Coxsackievirus A16 (CVA16), a member of the Enterovirus genus within the Picornaviridae family, is one of the major causative agents of hand, foot and mouth disease (HFMD) prevalent in infants and young children. Like other enteroviruses (EVs), CVA16 is a nonenveloped virus of ~30 nm in diameter with a single-stranded, positive-sense RNA genome of ~7.4 kb in length packaged in a protein shell termed capsid. Specifically, CVA16 utilizes cell surface heparan sulfate (HS) glycosaminoglycans as its attachment receptor, and human scavenger receptor B2 (SCARB2, also known as lysosomal integral membrane protein 2, LIMP-2) as its uncoating receptor. Cryo-EM studies show that 9B5 and 8C4 target distinct epitopes located at the 5-fold and 3-fold protrusions of CVA16 capsids, respectively, and exhibit differential binding preference to three forms of naturally occurring CVA16 particles.

From the same CVA16–8C4 dataset, we deduced three conformational states, namely C1, C2, and C3, at the resolution of 3.05, 2.91, and 3.36 Å and population distribution 15.5%, 27.0%, and 57.5%, respectively. For CVA16–8C4 C3, the radius of viral capsid is 170.5 Å, slightly larger than that of C1 and C2 (162.2 and 163.0 Å, respectively), and the two-fold axis channel in its capsid is open, while that in C1 and C2 capsid is closed. Moreover, the VP1 hydrophobic pocket is empty and collapsed in C3 capsid, but filled with the pocket factor in C1 and C2 capsids. Additionally, the viral RNA density is present in C1 but absent in C2 and C3. Collectively, these data suggested that the viral particles in C1, C2, and C3 adopt the native/compact mature CVA16 virion, the compact empty particle, and the expanded empty particle configuration, respectively. Moreover, structural comparison revealed that the protomers of the CVA16–8C4 C1/C2/C3 showed the most similar architecture to that of mature virion, compact empty particle, and expanded empty particle with the overall Cα RMSD values of 1.098, 1.178, and 0.937 Å, respectively, confirming the identity of these viral particles. It appears that 8C4 Fab binds only to the native mature virion (C1) and compact empty particle (C2), rather than the expanded empty particle (C3). In contrast, compared with CVA16-8C4 C1, CVA16-8C4 C3 displays a quite large upward movement for the expanded capsid and in particular an obvious outward tilting movement of up to 5.2 and 4.7 Å toward the Fab for the protomer 1 and protomer 2, respectively. Such a large movement toward the 8C4 Fab may create clashes between the CVA16 capsid and the 8C4 heavy chain, thus prevent 8C4 binding.

> GDPIADMIDQTVNNQVNRSLTALQVLPTAANTEASSHRLGTGVVPALQAAETGASSNASDKNLIETRCVLNHHSTQETAIGNFFSRAGLVSIITMPTMGTQNTDGYANWDIDLMGYAQLRRKCELFTYMRFDAEFTFVVAKPNGELVPQLLQYMYVPPGAPKPTSRDSFAWQTATNPSVFVKMTDPPAQVSVPFMSPASAYQWFYDGYPTFGEHLQANDLDYGQCPNNMMGTFSIRTVGTKKSPHSITLRVYMRIKHVRAWIPRPLRNQPYLFKTNPNYKGNDIKCTSTSRDKITTL;> SPSAEACGYSDRVAQLTIGNSTITTQEAANIVIAYGEWPEYCPDTDATAVDKPTRPDVSVNRFFTLDTKSWAKDSKGWYWKFPDVLTEVGVFGQNAQFHYLYRSGFCVHVQCNASKFHQGALLVAVLPEYVLGTIAGGTGNENSHPPYATTQPGQVGAVLTHPYVLDAGIPLSQLTVCPHQWINLRTNNCATIIVPYMNTVPFDSALNHCNFGLLVIPVVPLDFNAGATSEIPITVTIAPMCAEFAGLRQAVKQ;> GIPTELKPGTNQFLTTDDGVSAPILPGFHPTPPIHIPGEVRNLLEICRVETILEVNNLKTNETTPMQRLCFPVSVQSKTGELCAAFRADPGRDGPWQSTILGQLCRYYTQWSGSLEVTFMFAGSFMATGKMLIAYTPPGGSVPADRITAMLGTHVIWDFGLQSSVTLVVPWISNTHYRAHARAGYFDYYTTGIITIWYQTNYVVPIGAPTTAYIVALAAAQDNFTMKLCKDTEDIEQTANIQ>[10x]QANLMRLKSDLFNRSPMYPGPT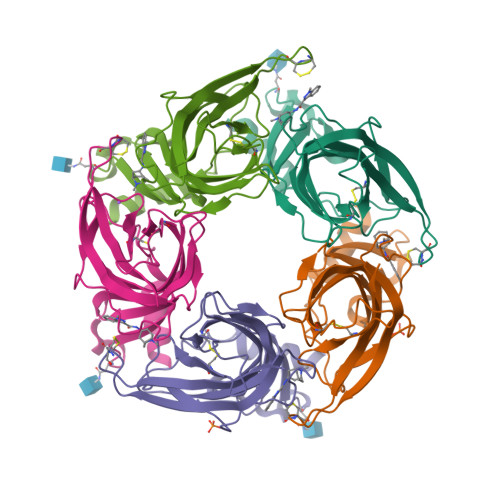KDDPLTVTLGFTLQDIVKVDSSTNEVDLVYWERQRWKLNSLMWDPNEYGNITDFRTSAADIWTPDITAYSSTRPVQVLSPQIAVVTHDGSVMFIPAQRLSFMCDPTGVDSEEGVTCAVKFGSWVYSGFEIDLKTDTDQVDLSSYYASSKYEILSATQTRQVQHYSCCPEPYIDVNLVVKFRER>HGYIKEPVSRAYMGALEKQTMGWTAAAQKYGSVIDNPQSVEGPKGFPAAGPPDGRIASANGGSGQIDFGLDKQTADHWVKQNIRGGFNTFTWHYTAPHATSKWHYYITKKNWNPNKPLSRDEFELIGTVNH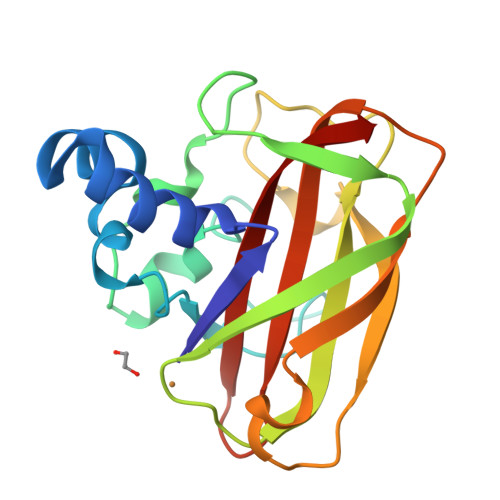DGSKADTNLTHKIFVPTDRSGYHIILGVWDVADTSNAFYNVIDVNLTK[2x]> TA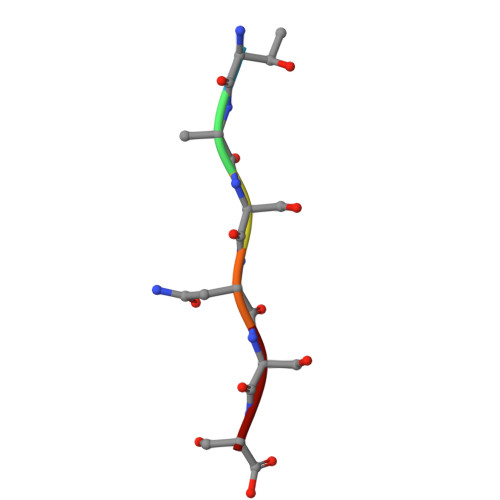SNSS D-galactonic acid | C6 H12 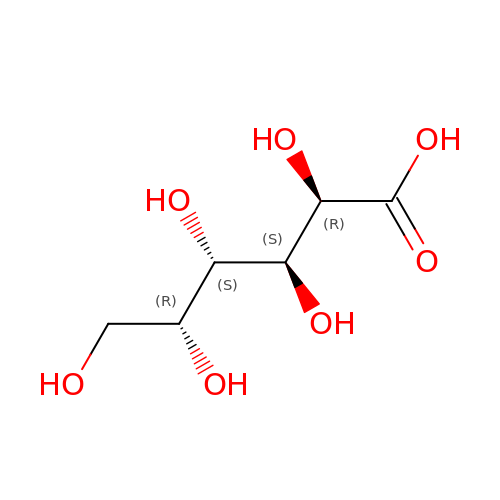O7 | RGHNJXZEOKUKBD-MGCNEYSASA-N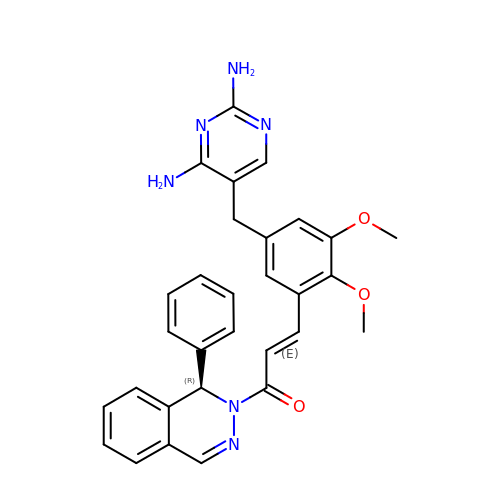(2E)-3-{5-[(2,4-diaminopyrimidin-5-yl)methyl]-2,3-dimethoxyphenyl}-1-[(1R)-1-phenylphthalazin-2(1H)-yl]prop-2-en-1-one | C30 H28 N6 O3 | NFQBNKYRVDDBSW-DBQZHCBRSA-N>MQKMLYFDDDVKQIVDHMFFKGFMFNDERIDRYFKESFTLRFLYREIGRQTVESFASQVLYITMTHEDYIYRVYGSDMYKYIEQVTDTQSQDLGKAIENAIEQGQTKDRQQDKGHEEYKDYEDTITKSFDDNRTAESTLPQSKVNIDVDNTVLDYADTNTISRDKNTSETVSEKTGTKDNTFDSLRNGESDTKRNTQSQNEMNRTGLTKQYLIDNLQKLYSMRDTIFKTYDKECFLHIW[2x];> MADRKLTHFKFFYNTPLTDYQNTIHFSSNNERDNYFLNENHFNAIDYKNIPFNFIRDRNMVNLEQMSWQDAQGINYCTFKSDFENRRYYAFVNQIEYVNDHVTRMYLVIDTVMTYTQGNVLSTVQNAFVERQHLPRDVYNYLLPSLRNNDDVIKASNKYYLNNYLEQFGGNLVLFQSSADLSKKFGTKKEPNLESSKGITYDYITSPVNLYVMNREDFNNFMDKMSKYPWITQNFQKIILIPATFINKDDLEAVKTQEDIKGLMTLKNDKLSNEWELKELRVPFERLQYMLNSNQDELKHLVRNEYLTIEIYSWNGDSLLLDAGKITERTGVKLKTKSIIGYHNEVRIYPVDYNSAPNEKPIKASDNSILIDTGSFLNTAITFDSFAEVPILIDNGLLAQSQQANKQKNAQSNLISNRINNVVNGNDLKSRFYDAVSIGSNLSPTALFSKFNDEYNYYKELRAEYKDLALQPPTVTSSQMGNAFQIANSINGLTMKIGVPAPFDMDNIQRYYFMLGFETNDQAGTPFPIDSWTVCNYLRMRGTYTIDGIDPMLLEQLKVLLETGVRFWHNDGTNNPMAQNVFKNKFRK

Staphylococcal picoviruses are a group of strictly lytic, short-tailed bacteriophages with compact genomes that are attractive candidates for therapeutic use. Here, we report the structure of the complete virion of S. epidermidis–infecting phage Andhra, determined using high-resolution cryo–electron microscopy, allowing atomic modeling of 11 capsid and tail proteins. The overall structure of the Andhra virion follows that of other phages in this group, with an isometric head (capsid) around 500 Å in diameter (vertex to vertex), connected to a 400-Å-long, straight tail surrounded by 12 appendages. The head has icosahedral symmetry, with the tail attached to a portal structure located at 1 of the 12 fivefold vertices.

Although the tail knob was expected to form a hexamer with C6 symmetry, it was inconsistently aligned relative to the RBPs, with two possible orientations, differing by a 30° rotation. We used symmetry expansion and 3D classification to generate a masked, focused reconstruction of this portion with only C3 symmetry, which was then resymmetrized to C6. The tail knob consists of a hollow cylinder, 145 Å long and 110 Å wide, and is made up of a hexamer of gp12. gp12 has a complex, intertwined structure that is similar to those of the gp9 tail knob protein of phage ϕ29 (45) and the streptococcal phage C1 major tail protein gp12 (46), to which it could be aligned with RMSD = 1.1 Å for 212 of the 588 residues. The N-terminal part of gp12 forms a β-sandwich domain related to tail tube proteins from many members of the Siphoviridae and Myoviridae bacteriophages, connected to an elongated β sheet domain at the bottom of the hexamer via an extended connecting loop. The polypeptide chain then returns to the top of the hexamer to complete the β sheet in the N-terminal domain. Residues 393 to 500 form an extended α-helical loop (the “channel loop”) on the inside of the cylinder, which constricts the inner diameter to ≈12 Å, presumably preventing exit of the DNA and terminal proteins. Most likely, these loops reorganize to become extruded through the tip of the tail during infection, enabling the resulting 12 α helices to insert into the host membrane to allow the passage of the DNA into the cell, similar to the mechanism proposed for ϕ29 (44). The focused reconstruction of the distal tail also resolved the hooks at the end of the β-hairpins of the tail stem protein (gp16) dodecamer that were not seen in the C6 reconstruction of the whole tail. Penetration of the membrane might cause the tail tip to fall apart, allowing the α helices of gp10 to disengage from the tail knob, leading to a conformational change in the internal α helices in the knob, similar to that described for ϕ29 (45).>MQIEVLIRNITPIFSAAPGSYYVSLDGTINPPQGASRFPLTRARTMTVVAETGDGVAKAVPLPIVPGNTMRNLLRRTMLKDVIEPALRDKSAQLSIGAYATAYAGNSSGNPDGVPSSFDEIVTMRAHPFLGLFGGGPRMLQGRLMVDSLYPIHQFSQRIIGSDYINDSIKGGITEIVWTRRNDPILQLGSPDDAAVIEGGAQAANDWITSLLATTKAKKGKAAKQADEAAESSDDNGRGLKAFNAHEVVIAGVKWLWRINVDRPSESQIGLILLALNKLANQRIAGGHAKDYGRFVIEDVILDGESVWTPSGVSGQATEQFFDAIAEALDGMTSSEFEQFAASAKEA[5x];> MDFLKVTINLGSPMVEPGDLFHLDALLGALRVSEVRAELGDGINPRDHHYDLPLEQYRSRSGQWVFKASAFHINKGAASQNWMQTSRINTAEAARHRSEGFLLLRAAKPNPAGGPFKNSLYHYPLVWATLTAYCVGDQARIADLLSQCRQIGGRRGVGCGRVAGFSVEVVPEVECTWALRAMPDDSEQSILCGEYALAMSALQSPYWDRSLHKPALVPTSLA;> MRYPSDVVDQVFKLPPDKGLLTWDNDPVACSHCARPIEKGDLYSPSSVGAFFSDTRNLASTSRSICWRCLILRKKQMLNGLSYALITQDGVFQISKDTNKAWLFTTPPPAPFFVMHSSSTMQHLCWRTPVTLDNRLIKVRYGNNLFVVRPEAIREALEIADRMNEGQKKWQAPIFLDRKAADSGHGALTKAGREHLSAADQEFLLNITPGERWALAYIMHSKRPQPEEPECITSKILEKL;> MFVTQVIFNMGERAYPDRARAMVAELMDGVQPGLVATLMNYIPGTSTSRTEFPTVQFGGASDGFCLLGFGDGGGAIVRDAVPLIHAALARRMPDRIIQVEHKEHSLSAEARPYVLSYTVPRMVVQKKQRHAERLLHEAEGKAHLEGLFLRSLQRQAAAVGLPLPENLEVEFKGAVGNFAAKHNPNSKVAYRGLRGAVFDVNARLGGIWTAGFMLSKGYGQFNATHQLSGAVNALSE

Type IV-A CRISPR-Cas systems diverge from this general mechanism, using a nuclease-independent interference pathway to suppress gene expression for gene regulation and plasmid competition. Here, we present several cryo-EM structures of two evolutionary distant type IV-A1 and type IV-A3 complexes (from Pseudomonas oleovorans and Klebsiella pneumoniae, respectively) bound to cognate DNA targets with and without DinG. The structures reveal multisubunit DNA-surveillance complexes that intimately recognize their DNA-targets to form an R-loop structure. Our results support a model in which DNA-binding is achieved analogously to type I Cascade, while recruitment of DinG differs mechanistically, even in closely related subtypes.

Cryo-EM structure determination of the resulting complexes revealed the effector complexes at average resolutions of ~3.0 Å (type IV-A1) and ~2.9 Å (type IV-A3). Five Cas7 subunits assemble a helical filament along the crRNA spine in type IV-A1, while six subunits form the Cas7-backbone in type IV-A3. In type IV-A1, the finger domain of Cas7.1 stabilizes the bipartite PAM interface while stacking against Cas5’s thumb motif and the Znf domain of Cas8. Cas8 inserts a short α-helix (α3) into the minor groove, with lysine 75 positioned near the A-T PAM base pairs at positions 1 and 2. On the opposite side, phenylalanine 51 aligns to the 5-methyl groups of the thymines in TS positions 1 and 2 of the PAM, stabilized by a short loop extending from the Cas5 thumb. Similarly, type IV-A1 Cas8 inserts a loop to stack the wedge residue threonine 120 against the PAM base pair in position 0. To deflect the TS for crRNA-mediated sequence interrogation, serine 119 of Cas8 and lysine 117 of Cas5 clamp the rotated phosphate that connects the PAM and dG1 of the TS. At the head of the type IV-A1 effector complex, Cas6 is recruited through its N-terminal RRM1 to the thumb of Cas7.4. Remarkably, the recruitment of Cas6 in this position caps the crRNA:TS hybrid by aligning the RRM domains via threonine 224 and histidine 225 against the terminal base pair formed between dG-28 (TS) and C28 (crRNA). In our P. oleovorans type IV-A1 structure, we could trace the single stranded NTS from the PAM to nucleotide 6, while the remaining NTS nucleotides were not visible, likely due to their flexibility.pyridin-2-ylboronic acid | C5 H6 B N O2 | 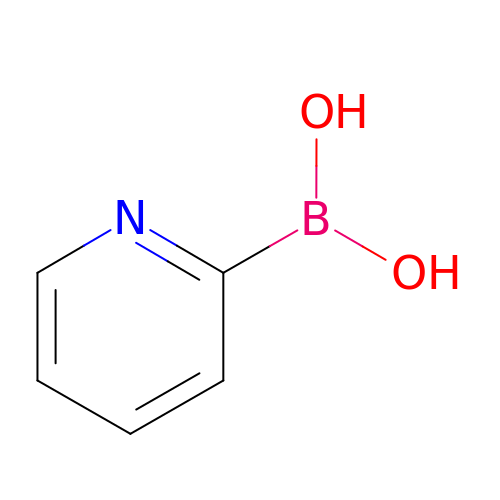UMLDUMMLRZFROX-UHFFFAOYSA-N> GGCUUAUCAAGAGAGGGGGAGUGACUGGCGCGAAGAACCCCGGCAACCAGAAAUGGUGCCAAUUCC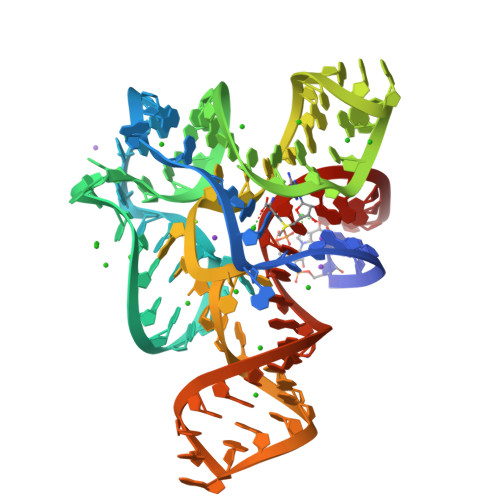UGCAGCGGAAACGUUGAAAGAUGAGCCG>[2x]GSHMKEINQTRDRLAKLNKELASSEQNKNHINNELKRKEEQLSSYEDKLFDVCGSQDFESDLDRLKEEIE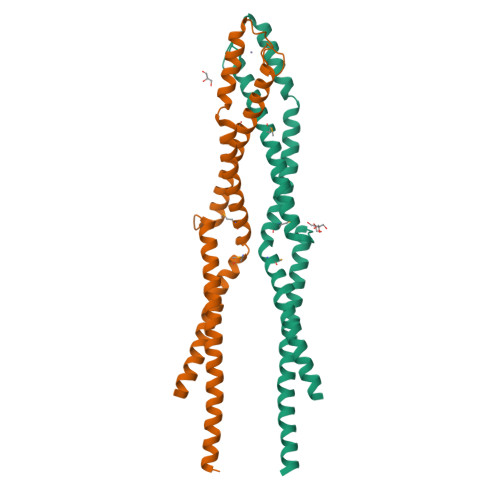KSSKQRAMLAGATAVYSQFITQLTDENQSCCPVCQRVFQTEAELQEVISDLQSKLRLAPDKLKSTESELKKKEKRRDEMLGLVPMRQSIIDLKEKEIPELRNKLQNVNRDIQRLKN> MKSNEHDDCQVTNPSTGHLFDLSSLSGRAGFTAAYSEKGLVYMSICGENENCPPGVGACFGQTRISVGKANKRLRYVDQVLQLVYKDGSPCPSKSGLSYKSVISFVCRPEAGPTNRPMLISLDKQTCTLFFSWHTPLACEQATECSVRNGSSIVDLSPLIHRTGGYEAYDESEDDASDTNPDFYINICQPLNPMHAVPCPAGAAVCKVPIDGPPIDIGRVAGPPI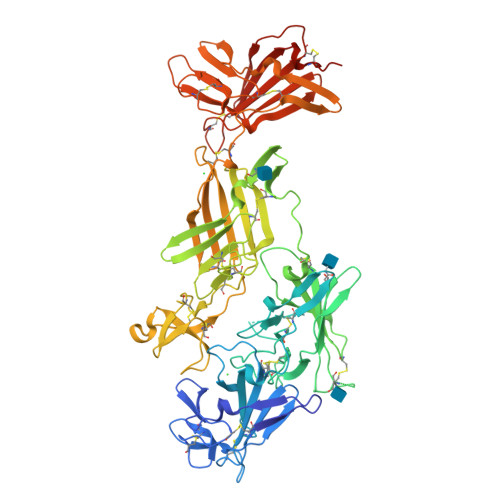LNPIANEIYLNFESSTPCLADKHFNYTSLIAFHCKRGVSMGTPKLLRTSECDFVFEWETPVVCPDEVRMDGCTLTDEQLLYSFNLSSLSTSTFKVTRDSRTYSVGVCTFAVGPEQGGCKDGGVCLLSGTKGASFGRLQSMKLDYRHQDEAVVLSYVNGDRCPPETDDGVPCVFPFIFNGKSYEECIIESRAKLWCSTTADYDRDHEWGFCRHSNSYRTSSIIFKCDEDEDIGRPQVFSEVRGCDVTFEWKTKVVCPPKKLECKFVQKHKTYDLRLLSSLTGSWSLVHNGVSYYINLCQKIYKGPLGCSERASICRRTTTGDVQVLGLVHTQKLGVIGDKVVVTYSKGYPCGGNKTASSVIELTCTKTVGRPAFKRFDIDSCTYYFSWDSRAACAVKHHHHHH>MAKTELSMGVASEDVTTLDPHFATTTSDRTLVSYIYGALVRFAPGSANPSSIEADLAESWESNADQLVWTFKLRPDVKWQGGYGNVTADDVVFSLDKARDPKRSAFSGDYAAIQKVEAVDAKTVRITLTRRVPSLLALLSNFSGGFIIPKKAFKERGDDFKRRPVGFGPFQVESIQPGQSVTLTANAEYFRGKPKLSKISYRFLNNEAARDLAFESGELDVEQGNQDQRWLQRLTANPENVVDTIEPAELNLLHINITKPPFNDIRVRQALAHTVNAAQIAKYRGERVNRAVPSVIPSNNLGFDPDAGVLNYDPAQSKKLLAEAGFPNGVTVTMVASQLPGLESLAQLIQAQVAE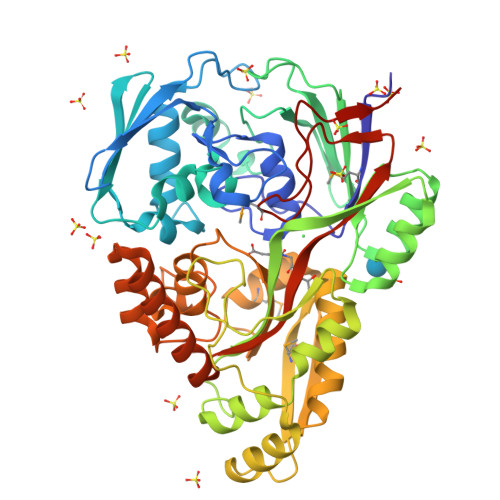GGFTLNLQPVEHAAWHQMIRKDLSPIVLYGAARFPIADYYLTQFYHSASEIGKPTQVVNFSHCNVADKQIEAARTETDPNKQIELWKEAQKLIVSNVCAIPLTENLGTWARKNKLGWGFELKGSMPSAPLITEQTYFKDHHHHHH[2x]propan-2-yl 4-indol-1-yl-4-oxidanylidene-butanoate | C15 H17 N O3 | 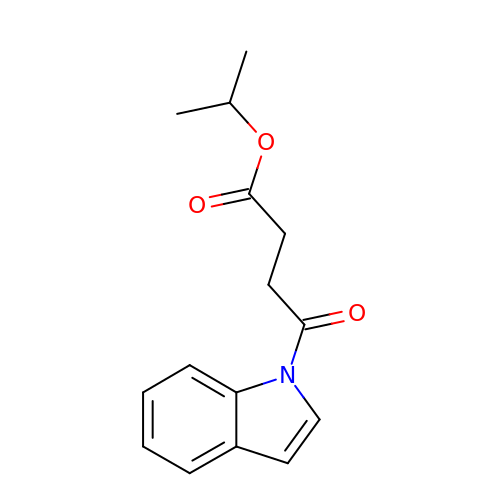VNSAQZLLFVPFAT-UHFFFAOYSA-N> MDPFEGRMTFLQLLGKLNASQFSQIKPAQFAIKHLDLEEDLYSCIWEELESGSFNTRVNIMYFVDTLCEMCLKNGLTGGYLNMISRDICKLVQNVAPIGAAGAANAPEVRKVLQSLHEKKVIDDNQYKDAMATVEAHE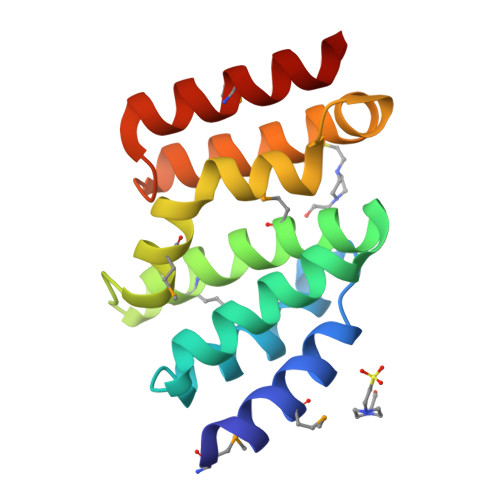QA> APKDNHHHHHHANKEATRNAAALFSVDYKAFLNEVDNLNKRMGDLRDINGEAGAWARIMSGTGSASGGFSDNYTHVQVGVDKKHELDGLDLFTGFTVTHTDSSASADVFSGKTKSVGAGLYASAMFDSGAYIDLIGKYVHHDNEYTATFAGLGTRDYSTHSWYAGAEAGYRYHVTEDAWIEPQAELVYGSVSGKQFAWKDQGMHLSMKDKDYNPLIGRTGVDVGKSFSGKDWKVTARAGLGYQFDLLANGETVLRDASGEKRIKGEKDSRMLMSVGLNAEIRDNVRFGLEFEKSAFGKYNVDNAVNANFRY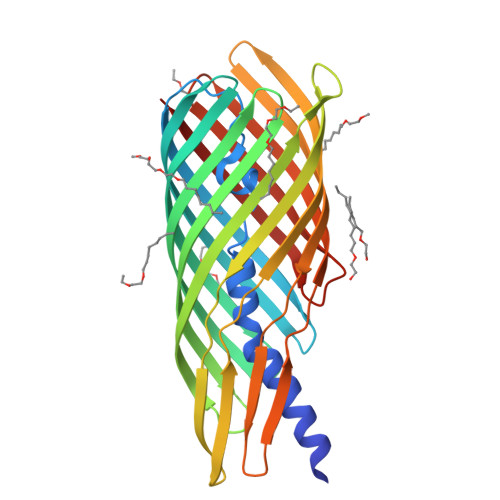SF>[2x]MRLATIRTNGTTIAARVESENTATTIEGFANVGELLQESNWRELAENAAGEAVTFENKELDAVVPAPKKIVCVGLNYANHIKEMGRDLPDTPTLFVKFPDALIGPFDDVVVPEWANKALDWEGEMAVIIGKRARRVKQADAAEYIAGYAVMNDYTTRDFQYAAPAKTPQWH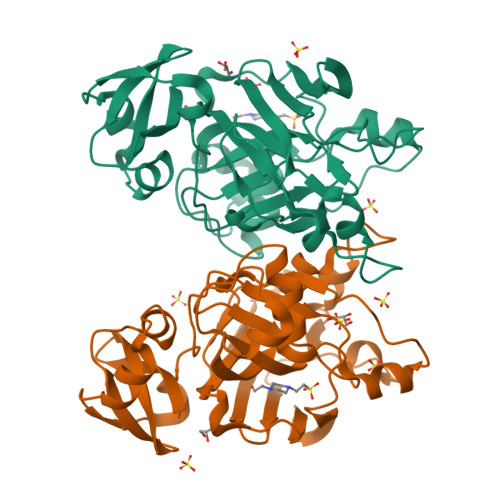QGKSLEKSAGFGPWMTTPDSFEFGGELATYLEGEKVQSTPTNDLVFSPEKLIEYITHIYPLDAGDVIVTGTPGGVGHARNPQRYIGDGETVKVEIAGLGFIENKTVFELEHHHHHH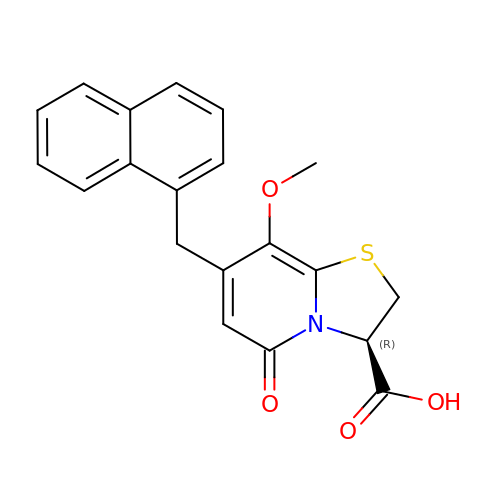(3~{R})-8-methoxy-7-(naphthalen-1-ylmethyl)-5-oxidanylidene-2,3-dihydro-[1,3]thiazolo[3,2-a]pyridine-3-carboxylic acid | C20 H17 N O4 S | PPMCZEBJGJNUJF-INIZCTEOSA-N>[2x]MSELTHPTIVDGWFREISDTMWPGQAMTLRVEKILHHEKSKYQDVLVFKSTDYGNVLVLDNAIQVTERDEFSYQEMIAHLALNSHPNPKKVLVIGGGDGGVLREIVKHDSVQEAWLCDIDEA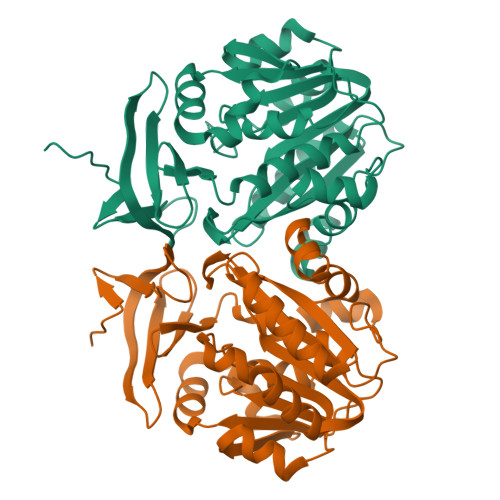VIRVSKEYLPEMAKSYSHPKVKTHIGDGFQFLRDYQNTFDVIITDSSDPEGPAASLFQQSYFELLNGALTEKGVISTQAESMWIHLPIIKELKKACKEVFPTVGYAYTTIPTYPTGQIGFMVCSKDANVDVTKPLRSISEEEEEAKYRYYNKKVHEASFVLPTWVAKELDL>TITEWS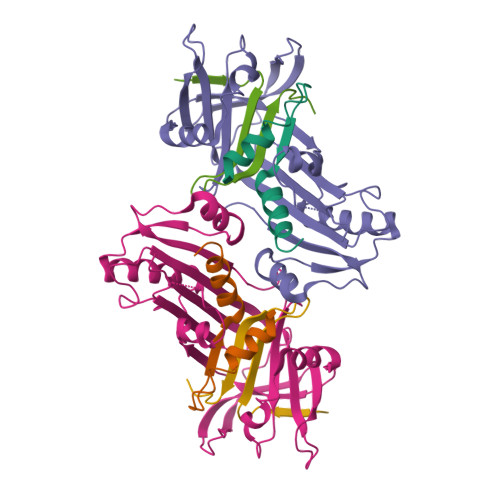VNMYNHLRGTGEDENILFSPLSIALAMGMMELGA[2x];>ENQYVMKLANSLFVQNGFHVNEEFLQMLKMYFNAEVNHVDFSQNVAVANSINKWVENYTNSLLKDLVSPEDFDGVTNLALINAVYFKGNWKSQFRPENTRTFSFTKDDESEVQIPMMYQQGEFYYGEFSDGSNEAGGIYQVLEIPYEGDEISMMLALSRQEVPLATLEPLLKAQLIEEWANSVKKQKVEVYLPRFTVEQEIDLKDILKALGVTEIFIKDANLTAMSDKKELFLSKAVHKSCIEVNEEGSEAAAASGMIAIS[2x];>YPQVIVDHPFLYLIRNRKSGIILFMGRVMNPHH[2x]> GPGNEVTLLDSRSVQGELGWIASPLEGGWEEVSIMDEKNTPIRTYQVCNVMEPSQNNWLRTDWITREGAQRVYIEIKFTLRDCNSLPGVMGTCKETFNLYYYESDNDKERFIRENQFVKIDTIAADESFTQVDIGDRIMKLNTEIRDVG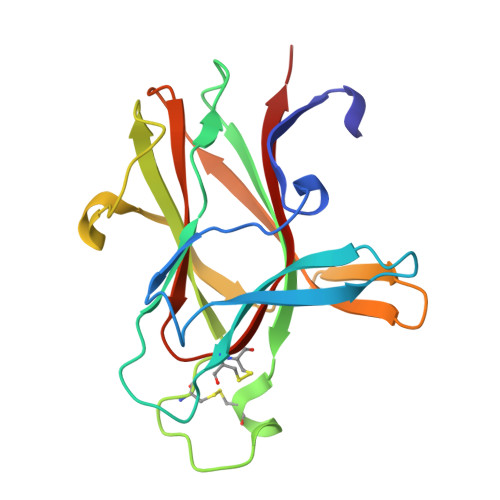PLSKKGFYLAFQDVGACIALVSVRVFYKKA> MVPEVFAQARLRMDQLTKPPRALGYLEEVALRLAALQGRVKPELGRGAVVVAAADHGVVAEGVSAYPQEVTRQMVLNFLRGGAAINQFALAADCAVYVLDVGVVGELPDHPGLLKRKVRPGTANLAQGPAMTPEEAERALLAGREAARRAIAEGATLLAAGDMGIGNTTAAAALTAALLGLPPEAVVGRGTGVGEEGLRRKRQAVARALARLHPGMGPLEVAAEVGGIELVAIAGIYLEGYEAGLPLVLDGFPVTAGALLAWK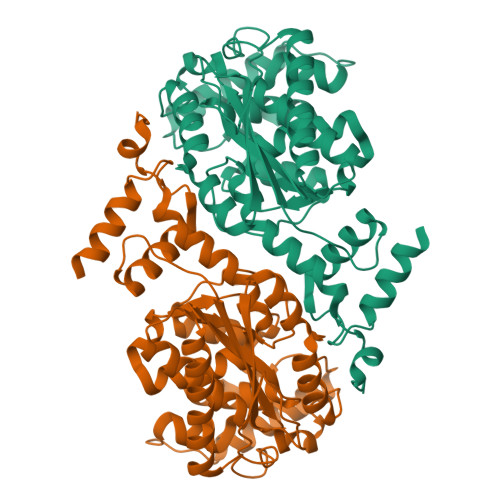MAPGLRDHLFAGHLSREPGHRHQLEALGLRPLLDLDLALGEGTGAVLAMPLLRAAARILHMATFQEAGVSRG>[2x]MASNSLEIEELARFAVDEHN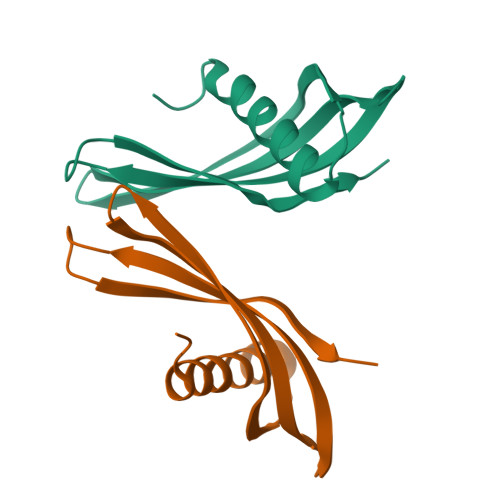KKENALLEFVRVVKAKEQANLYLSTPIDTMYYLTLEAKDGGKKKLYEAKVWVKHIMYYPKTANFKELQEFKPVGDAAAAHHHHHHHH> GPAKQYDSVECPFCDEVSKYEKLAKIGQGTFGEVFKARHRKTGQKVALKKVLMENEKEGFPITALREIKILQLLKHENVVNLIEICRTKASPYNRCKGSIYLVFDFCEHDLAGLLSNVLVKFTLSEIKRVMQMLLNGLYYIHRNKILHRDMKAANVLITRDGVLKLADFGLARAFSLAKNSQPNRYTNRVVTLWYRPPELLLGERDYGPPIDLWGAGCIMAEMWTRSPIMQGNTEQHQLALISQLCGSITPEVWPNVDNYELYEKLELVKGQKRKVKDRLKAYVRDPYALD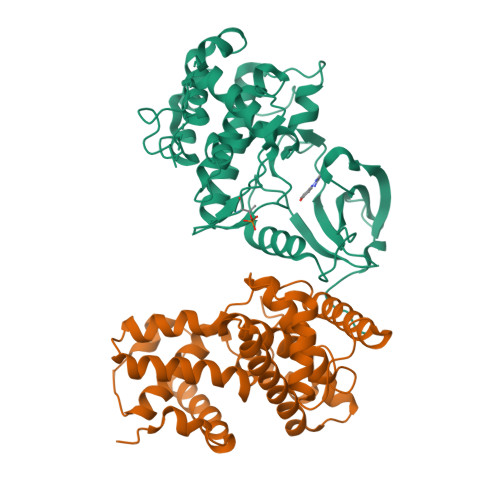LIDKLLVLDPAQRIDSDDALNHDFFWSDPMPSDLKGMLST;> MEGERKNNNKRWYFTREQLENSPSRRFGVDPDKELSYRQQAANLLQDMGQRLNVSQLTINTAIVYMHRFYMIQSFTQFPGNSVAPAALFLAAKVEEQPKKLEHVIKVAHTCLHPQESLPDTRSEAYLQQVQDLVILESIILQTLGFELTIDHPHTHVVKCTQLVRASKDLAQTSYFMATNSLHLTTFSLQYTPPVVACVCIHLACKWSNWEIPVSTDGKHWWEYVDATVTLELLDELTHELLQILEKTPNRLKRIWNWR>MSRLDKSKVINSALELLNEVGIEGLTTRKLAQKLGVEQPTLYWHVKNKRALLDALAVEILARHKDYSLPAAGESWQSFLRNNAMSFRRALLRYRDGAKVHLGTRPDEKQYDTVETQLRFMTENGFSLRDGLYAILAVIHFTLGAVLEQQEHTAALTDRPAAPDENLPP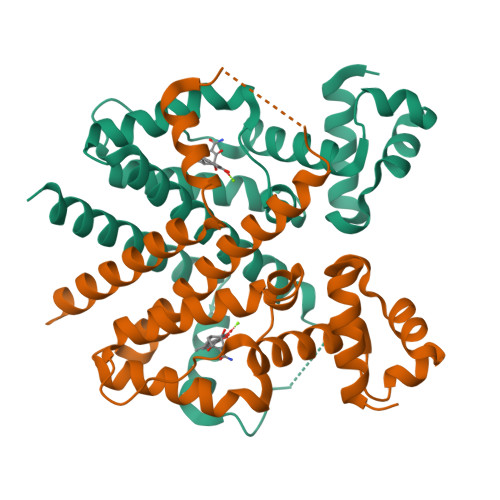LLREALQIMDSDDGEQAFLHGLESLIRGFEVQLTALLQIV[2x]> AMLPISMSDEGDSFLVKDSLGENKIPKNPSKVVILDLGILDTFDALKLNDKVVGVPAKNLPKYLQQFKNKPSVGGVQQVDFEAINALKPDLIIISGRQSKFYDKLKEIAPTLFVGLDNANFLSSFENNVLSVAKLYGLEKEALEKISDIKNEIEKAKSIVDEDKKALIILTNSNKISAFGPQSRFGIIHDVLGINAVDENIKVGTHGKSINSEFILEKNPDYIFVVDRNVILGNKERAQGILDNALVAKTKAAQNKKIIYLDPEYWFLASGNGLESLKTMILEIKNAVK

The periplasmic binding protein (PBP) CeuE1 is an important component of the Fe(III) uptake system in Campylobacter jejuni, a commensal Gram-negative bacterium in the avian gut, but a common source of food poisoning in humans. CeuE, an integral part of the CeuBCDE ABC transporter of C. jejuni, is responsible for capturing Fe(III)-siderophore complexes in the periplasm for delivery to their respective inner membrane transporter. C. jejuni does not itself synthesize siderophores, but capitalizes on their secretion by other bacteria, such as E. coli. Here we report a combined solution and structural study of a series of synthetic tetradentate analogues of the enterobactin-derived bis(2, 3-dihydroxybenzoyl-L-Ser), to explore the ligand-binding promiscuity of CeuE, both wild type and with mutations of the Fe(III) binding residues H227 and Y288.

To probe the relative contributions of His227 and Tyr288 to Fe(III)-siderophore binding, site-directed mutagenesis was then used to replace the side chains of the two Fe(III)-coordinating amino acids with non-coordinating side chains of similar size. His227 was mutated to either leucine (H227L) or alanine (H227A), while Y288 was mutated to phenylalanine (Y288F). All five mutants (Y288F, H227L, H227A, H227L/Y288F, H227A/Y288F) were crystallized in their apo form, and all structures are closely similar to that of wild type CeuE. However while there is clear electron density for the Y288F mutation in its three structures, H227L and H227A are located in a flexible loop region and there is generally no electron density to confirm their presence. Mutation of the Fe(III)-coordinating tyrosine led to a drastic drop in binding affinity in both the single (Y228F) and the double mutants (H227L/Y288F and H227A/Y288F), with Kd values above 1 μM. Site-directed mutagenesis of CeuE revealed that Y288 is essential for binding, as the binding affinity observed in the fluorescence titration experiments is far weaker for all mutants containing Y228F when compared to the wild type protein. This finding is confirmed by the lack of CD signal corresponding to the Λ-configuration when Fe-5-Lic is added to these mutants. The Y228F mutants gave no signal, confirming a lack of Λ-configuration induction, which may indicate a lack of ligand binding.> GAKSIYEFQVNAADGKPYDLSQHKGHPLLIYNVASRCGYTKGGYETATTLYNKYKGQGFTVLAFPCNQFAGQEPGTALEVKEFACTRFKADFPIMAKIDVNGSKAHPLYEFMKA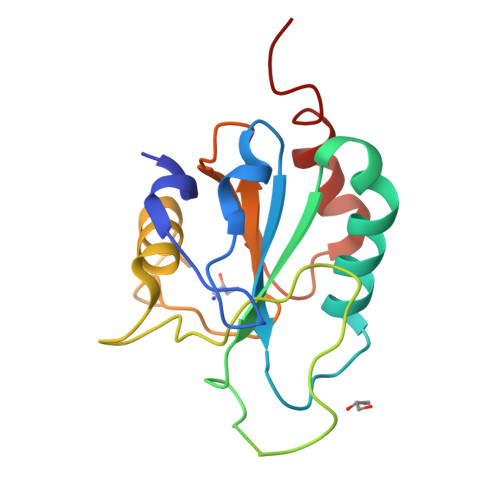TIPGLFGTKAIKWNFTSFLIDRHGVPVERFSPGASVEDIEKKLLPLLGGARI>[2x]MTAPFAIRRLNAADPDFGRHLDHLLSWESVSDDSVNQRVLDIIAAVRSRGDAAVVEFTQRFDGLQAASMADLILPRERLELALTRITVAQREALEVAAERVRSYHEKQKQGSWRYTEADGTVLGQQVTPLDRAGLYVPGGKA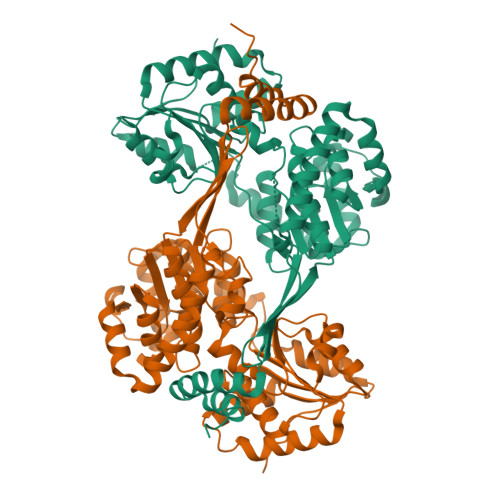SYPSSVLMNAIPAKVAGVSEVVMVVPTPRGEINEIVLAAACIAGVDRVFTIGGAQAVAALAYGTESVPRVDKIVGPGNIYVATAKRHVFGQVGIDMIAGPSEILVVCDGQTDPDWIAMDLFSQAEHDEDAQSILVSPDAAFLDRVADSIARLLPTMERAEIIRTSLEGRGALIQVADQAQACAVANRIAPEHLELSVADPESWLPEIRHAGAIFMGRYTAEALGDYCAGPNHVLPTSGTARFSSPLGVYDFQKRSSIINCSAEGASVLGRTASVLARGESLTAHARSAEYRILDEKEA> MDEFEMIKRNTSEIISEEELREVLKKDEKSAHIGFEPSGKIHLGHYLQIKKMIDLQNAGFDIIILLADLAAYLNQKGELDEIRKIGDYNK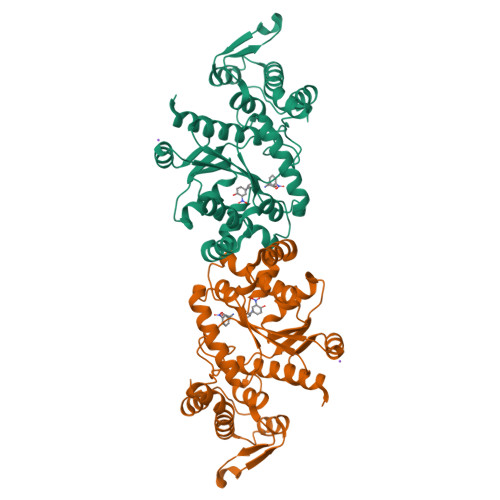KVFEAMGLKAKYVYGSEFQLDKDYTLNVYRLALKTTLKRARRSMELIAREDENPKVAEVIYPIMQVNCAHYRGVDVAVGGMEQRKIHMLARELLPKKVVCIHNPVLTGLDGEGKMSSSKGNFIAVDDSPEEIRAKIKKAYCPAGVVEGNPIMEIAKYFLEYPLTIKRPEKFGGDLTVNSYEELESLFKNKELHPMDLKNAVAEELIKILEPIRKRLLEHHHHHH> MPKPYIAINMADLKNEPKTFEMFSAVGPKVCMVTARHPGFVGFQNHVQIGVLPFGERFGGAKMDMTKESSTVRVLQYTMWKDWKDHEEMHRQNWSYLFRLCYSCASQMVWGPWEPIYEIKYADMPINTEMTDFTAVVGKKFAEGKPLEIPVISQPYGKRVVAFGEHTVIPGKEEQFEDAIIKTLEMFKRAPGFLGAMLLKEIGVSGIGSFQFGSKGFHQLLESPGSLEPDPNNVMYQAPEAKPTPP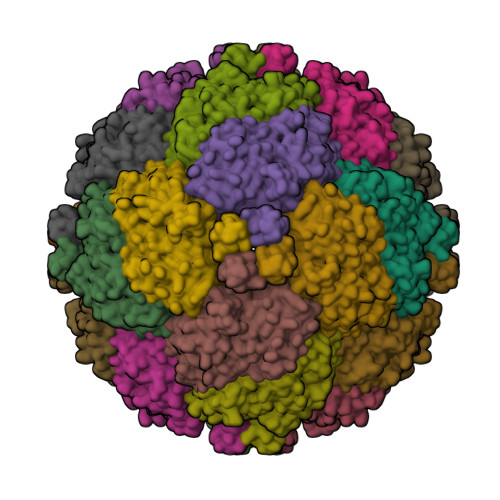QYIVHVEWANLDALQFGMGRVLLSPEYREVHDEALDTLIYGPYIRIINPVMEGTFWREYLNE6-(2-{3-[3-(dimethylamino)propyl]-2,6-difluorophenyl}ethyl)-4-methylpyridin-2-amine | 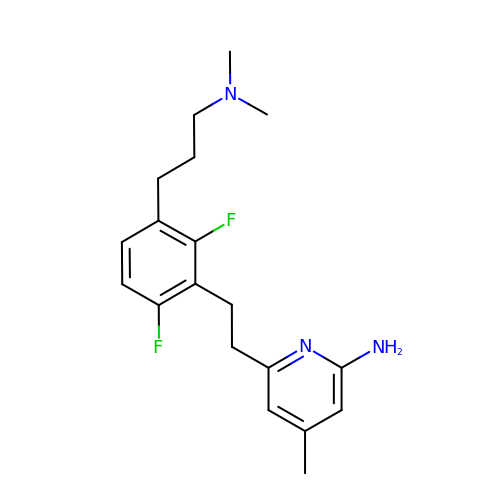C19 H25 F2 N3 | MXQLPMXQTGKLHB-UHFFFAOYSA-N>MFPTGWRPKLSESIAASRMLWQPMAAVAVVQIGLLWFSPPVWGQDMVSPPPPIADEPLTVNTGIYLIECYSLDDKAETFKVNAFLSLSWKDRRLAFDPVRSGVRVKTYEPEAIWIPEIRFVNVENARDADVVDISVSPDGTVQYLERFSARVLSPLDFRRYPFDSQTLHIYLIVRSVDTRNIVLAVDLEKVGKNDDVFLTGWDIESFTAVVKPANFALEDRLESKLDYQLRISRQYFSYIPNIILPMLFILFISWTAFWSTSYEANVTLVVSTLIAHIAFNILVETNLPKTPYMTYTGAIIFMIYLFYFVAVIEVTVQHYLKVESQPARAASITRASRIAFPVVFLLANIILAFLFFGF[5x]

GLIC is a bacterial homologue of the pentameric ligand-gated ion channels (pLGICs) that mediate the fast chemical neurotransmission of nerve signalling in eukaryotes. Because the activation and allosteric modulation features are conserved among prokaryotic and eukaryotic pLGICs, GLIC is commonly used as a model to study the allosteric transition and structural pharmacology of pLGICs. Unlike the other pLGICs, GLIC displays a particular activation mechanism in which protons, rather than a sizable agonist, trigger ion-channel opening. Here, experimental evidence for carboxylate binding to GLIC is provided by solving its X-ray structures with a series of monocarboxylate and dicarboxylate derivatives, and two carboxylate-binding sites are described: (i) the ‘intersubunit’ site that partially overlaps the canonical pLGIC orthosteric site and (ii) the ‘intrasubunit’ vestibular site, which is only occupied by a subset of the described derivatives.

In attempt to check whether other dicarboxylic acids with different lengths are also able to bind GLIC, we solved crystal structures of GLIC in complex with malonate (diC3) and glutarate (diC5) at 2.9 and 2.65 Å resolution, respectively. The first carboxylic groups of malonate and glutarate occupied the position of acetate, with a similar interaction pattern with Arg77, Glu181 and Arg105. Indeed, all of the monocarboxylic and dicarboxylic acids were found to bind in this pocket with a similar binding mode for the first carboxylic group involving Arg77 and Glu181 from one subunit and Arg105 from the neighbouring sububnit. For dicarboxylates, except for malonate, Asn152 from the complementary subunit contributes to the coordination of the second carboxylic group.> EEIRPKEVYLDRKLLTLEDKELGSGNFGTVKKGYYQMKKVVKTVAVKILKNEANDPALKDELLAEANVMQQLDNPYIVRMIGICEAESWMLVMEMAELGPLNKYLQQNRHVKDKNIIELVHQVSMGMKYLEESNFVHRDLAARNVLLVTQHYAKISDFGL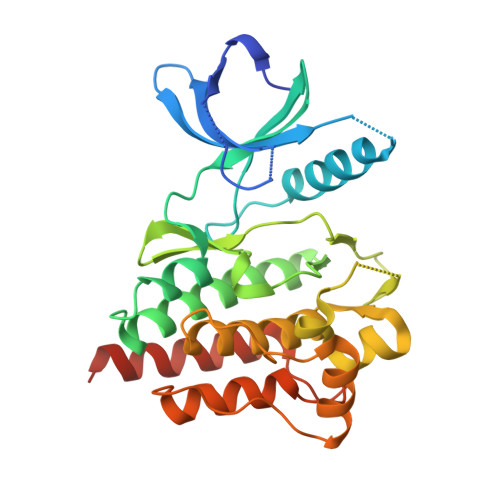SKALRADENYYKAQTHGKWPVKWYAPECINYYKFSSKSDVWSFGVLMWEAFSYGQKPYRGMKGSEVTAMLEKGERMGCPAGCPREMYDLMNLCWTYDVENRPGFAAVELRLRNYYYDVVNLEHHHHHHHH Here, we report on incorporating an N-tert-butylguanidinium group at the 2′,4′-bridging structure, which greatly enhances duplex-forming ability because of its interactions with the minor groove. X-ray crystal structures of the self-complementary GuNA[Me,Me]- and GuNA[Me,tBu]-modified oligonucleotides showed that interactions between the N-tert-butyl group and the minor groove greatly enhanced the duplex stability. Two self-complementary sequences were selected; (1) a 10 mer oligodeoxynucleotide (5′-GCGTATACGC-3′)(35) and (2) an 8 mer oligodeoxynucleotide (5′-GTGBrUACAC-3′), where BrU represents a 5-bromourasil nucleobase(43)—these sequences have been used previously for crystallographic analysis. All three crystal structures were found to adopt the A-form duplex.

Among them, three oligonucleotides, ODN25, ODN28 and ODN29, formed good crystals for X-ray crystallographic analysis, and their crystal structures were successfully determined at the resolutions of 2.01, 0.95 and 0.93 Å, respectively. On the other hand, two tert-butyl groups of the duplexed ODN29 were located on the minor groove side, and two GuNA[Me,tBu]s were found to have similar structures. Notably, we found that the tert-butyl-substituted guanidine moiety and the 2-carbonyl group of the thymine nucleobase formed a hydrogen bond (3.4 Å for ODN25 in Figure 3C and 3.2 Å for ODN29 in Figure 4B), suggesting that this additional hydrogen-bond contact, as well as the hydrophobic interactions between the tert-butyl group and the minor groove, contributed greatly to duplex stability. GuNA[Me,Me] and GuNA[Me,tBu] had different hydrogen-bond distances in their T•A base pairs (N3(T)–N1(A): 2.9 Å for GuNA[Me,Me] and 2.7 Å for GuNA[Me,tBu]; O4(T)–N6(A): 2.9 Å for GuNA[Me,Me] and 3.1 Å for GuNA[Me,tBu]). Shortened N3(T)–N1(A) bonds were observed when the tert-butyl group was tightly bound to the minor groove. Using space-filling models, we confirmed that the tert-butyl groups fit tight into the minor groove. Similarly, ODN29 bearing GuNA[Me,tBu] at the second position from the 5′-end exhibited a much higher Tm (55°C) than the corresponding GuNA[Me,Me]-modified oligonucleotide (44°C for ODN28). Taken together, the increased duplex stability can be understood by the following three processes: (i) the tert-butyl group of GuNA[tBu] or GuNA[Me,tBu] bound tightly to the minor groove, (ii) an additional hydrogen bond formed, and (iii) the nearby T•A base-pair strengthened. In these three X-ray crystal structures, no counter anion was observed around the guanidium part.

> GXGUACAC Magnesium chelatase is a conserved enzyme complex responsible for the first committed step of chlorophyll biosynthesis in photosynthetic organisms, which is the addition of magnesium to the chlorophyll precursor, protoporphyrin IX. The complex is composed of the catalytic subunit ChlH, the bridging subunit ChlD, and the subunit ChlI, which serves as the motor that drives the entire complex. The motor subunit ChlI belongs to the superfamily of AAA+ (ATPases associated with diverse cellular activities) proteins and, through binding and hydrolyzing of ATP, provides the energy for the thermodynamically unfavorable reaction of Mg2+ insertion into protoporphyrin IX. Here, we used a combination of cryo-EM and functional analysis to investigate the mechanism of the ChlI motor subunit of magnesium chelatase from the cyanobacterium Nostoc sp. PCC 7120 (hereafter, Nostoc).

Our 3D classifications revealed a class corresponding to a pentameric structure of ChlI, which we attribute to an intermediate state of ChlI complex formation. The map reached an overall resolution of 4.9 Å and differs significantly from the hexamer maps. The ChlI pentamer shows a spring-washer-like helical organization with an opening of approximately 45 Å between the first and last monomers in the complex, which would be sufficient to accommodate an additional monomer of ChlI. The resolution obtained for this structure allowed for the fitting of α-helices and β-strands of ChlI monomers but restricted the accurate determination of bound nucleotide molecules. However, the cryo-EM density obtained contains areas that are not occupied by the polypeptide chain of the ChlI protein and are close to the nucleotide binding pocket (insets 1–4). Therefore, we suggest that the ChlI pentamer carries at least four nucleotide molecules that we, however, could not unambiguously assign to ATP or ADP. The three central monomers of the pentamer contain partially folded insertions and generally show higher local resolution. In contrast, the two peripheral monomers are less resolved, possibly due to the increased flexibility of the ChlI pentamer at its ends. Of note, our pentameric structure of ChlI also contains nucleotide molecules bound between adjacent monomers, supporting the model that ChlI requires ATP for oligomerization. The oligomers then grow and form helical spring-washer-like pentameric structures, potentially representing a resting state of the enzyme, similar to the Lon protease’s open helical state or the AAA+ protein RavA, which creates a mix of open spiral and closed planar ring state populations.

>[5x]MHHHHHHTPTAQTTASARRVVFPFTAIVGQEEMKLALLLNVIDPKIGGVMIMGDRGTGKSTTIRALADLLPEIPVVANDPFNSDPSDPDLMSDEVRQKSGTGAEIPIEFKKVQMVDLPLGATEDRVCGTIDIEKALSEGVKAFEPGLLAKANRGILYVDEVNLLDDHLVDVLLDSAASGWNTVEREGISIRHPARFVLVGSGNPEEGELRPQLLDRFGMHAEIHTVKEPALRVQIVEQRSEFDQNPPTFLEKYNPEQTALQKKIVEAQKLLPEVKLDYDLRVKISEVCSELDVDGLRGDIVTNRAAKALTAYEGRTEVTVDDIRRVITLCLRHRLRKDPLESIDSGYKVEKVFARIFGVELLEDDSSQKNGAGQIKTGVR>MAKMRISPELKKLIEKYRCVKDTEGMSPAKVYKLVGENENLYLKMTDSRYKGTTYDVEREKDMMLWLEGKLPVPKVLHFERHDGWSNLLMSEADGVLCSEEYEDEQSPEKIIELYAECIRLFHSIDISDCPYTNSLDSRLAELDYLLNNDLADVDCENWEEDTPFKDPRELYDFLKTEKPEEELVFSHGDLGDSNIFVKDGKVSGFIDLGRSGRADKWYDIAFCVRSIREDIGEEQYVELFFDLLGIKPDWEKIKYYILLDELF[2x]

For aminoglycosides, a group of antibiotics used to treat serious nosocomial infections, the main mechanism of resistance is via the enzymatic inactivation of the drug by acetyltransferases, nucleotidyltransferases, or phosphotransferases. Among the three types of aminoglycoside-modifying enzymes, aminoglycoside phosphotransferases or kinases (APHs) yield the highest levels of resistance thereby providing a rationale for focusing inhibitor development for these specific resistance factors. Combined, these studies reveal that although members of the APH family share low similarities in sequence and their ligand specificity varies greatly, their overall three-dimensional fold is homologous to each other and to that of ePKs. To further examine the suitability of the CKI-7 scaffold for inhibitor development, we determined the crystal structures of APH(3′)-IIIa and APH(9)-Ia in complex with CKI-7.

Previously, details on the inhibition of APH(3′)-IIIa by CKI-7 have been reported (Ki = 66.1±7.5 µM). The APH(3′)-IIIa-CKI-7 inhibitor complex was crystallized in the space group P212121 with two inhibitor-bound enzyme molecules in the asymmetric unit, analogous to the nucleotide bound enzyme complexes. The structure has been refined to 2.15 Å with an Rcryst of 0.189 and Rfree of 0.235. In the nucleotide-bound enzyme structures, the loop is positioned above the phosphate moieties of the nucleotide, whereas, in the APH(3′)-IIIa-CKI-7 structure, the tip of the loop points back into the phosphate-binding area, delimiting the nucleotide-binding pocket, reminiscent of what is seen in the apo state of APH(3′)-IIIa. A principal contact between the isoquinoline or adenine ring with APH is the stacking interactions conferred by the aromatic ring side chain of Tyr42 in APH(3′)-IIIa and Phe50 in APH(9)-Ia. Consequently, an interaction analogous to that between N1 of the adenine and the linker amide is observed between N2 of the isoquinoline and the amide of Ala93 in APH(3′)-IIIa or Ile103 in APH(9)-Ia. In APH(3′)-IIIa, the aminoethyl-amide adopts an extended conformation and it is situated just beyond the ribose-binding area, toward the solvent exposed opening of the ATP-binding pocket. Two hydrogen bonds are observed between this section of the CKI-7 and the APH(3′)-IIIa. One of which is found between one of the oxygen atoms of the sulfonyl group (O2S) and the hydroxyl group of Tyr42. The second hydrogen bond is formed between the terminal nitrogen of the aminoethyl tail, N2′, and the main chain carbonyl of Ser194.> GMASLPKRIIKETEKLVSDPVPGITAEPHDDNLRYFQVTIEGPEQSPYED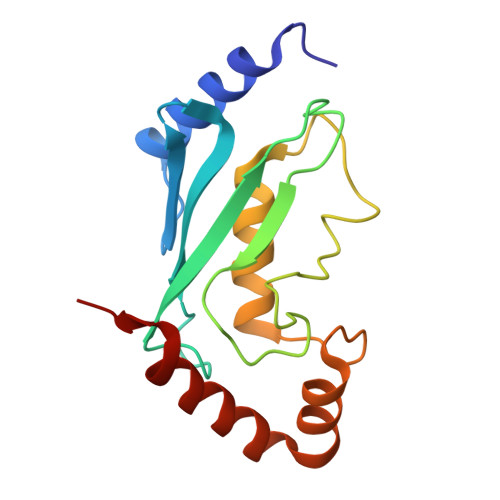GIFELELYLPDDYPMEAPKVRFLTKIYHPNIDRLGRICLDVLKTNWSPALQIRTVLLSIQALLASPNPNDPLANDVAEDWIKNEQGAKAKAREWTKLYAKKKP>MASGMIVTDAGADQPIVFVNRAFSTITGYAPNEVLGRNARFLQGPQTDAATVARLREAIAAARPIQERILNYRKDGQPFWNQLSISPVRDETGNVVAFVGVKTDVTAHHHHHH[2x]

Flavin-binding fluorescent proteins (FbFPs), engineered from prokaryotic and eukaryotic light, oxygen, voltage (LOV) photoreceptors, are promising fluorescent reporter proteins. Their small size (about 10 kDa for monomeric FbFPs such as the improved LOV (iLOV) protein derived from Arabidopsis thaliana phototropin photoreceptors) and their oxygen-independent fluorescence make them ideal reporters to monitor transport and anaerobic biological processes. In contrast to GFP-like fluorescent reporter proteins, whose absorption and fluorescence maxima can be tuned by exchanging certain chromophore-constituting amino acids, the absorption and fluorescence of FbFPs and other flavoproteins depends on noncovalently bound flavins, whose structure cannot be influenced by mutation. Using spectroscopy, X-ray crystallography, and quantum mechanics molecular mechanics calculations, we provide a firm structural and functional understanding of spectral tuning in FbFPs.

To verify the transferability of the blue-shifting Q489K mutation, identified for the plant FbFP iLOV, we introduced the corresponding Q148K mutation into the recently presented thermostable CagFbFP protein from thermophilic phototrophic bacterium Chloroflexus aggregans. Much like iLOV–Q489K, CagFbFP–Q148K possesses a blue-shifted S0→S1 absorption band with a maximum at around 444 nm (≈3 nm blue-shifted relative to parental CagFbFP) and a blue-shifted fluorescence-emission maximum (≈6 nm blue shift relative to parental CagFbFP; compare the gray dashed line and solid blue line). To verify that the structural changes, which we observed for iLOV–Q489K, are indeed a consequence of the introduced Q489K mutation and are not due to the observed succinimide modification, we obtained the structure of the corresponding CagFbFP–Q148K variant. Altogether, we were able to obtain three types of CagFbFP–Q148K crystals, all using the precipitant solutions with pH of 6.5 (data and refinement statistics are summarized in Table S1). In all of the obtained models, the C terminus of the protein is clearly unlatched, and the side chain of the introduced lysine is facing away from FMN as was found in iLOV–Q489K. The photophysical properties of the CagFbFP variants are relatively straightforward to interpret.> FPTDDDDKIVGGYTCAANSIPYQVSLNSGSHFCGGSLINSQWVVSAAHCYKSRIQVRLGEHNIDVLEGNEQFINAAKIITHPNFNGNTLDNDIMLIKLSSPATLNSRVATVSLPRSCAAAGTECLISGWGNTKSSGSSYPSL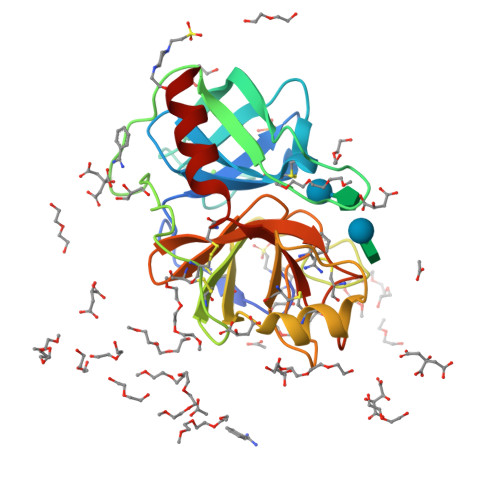LQCLKAPVLSDSSCKSSYPGQITGNMICVGFLEGGKDSCQGDSGGPVVCNGQLQGIVSWGYGCAQKNKPGVYTKVCNYVNWIQQTIAAN> FDLNDFL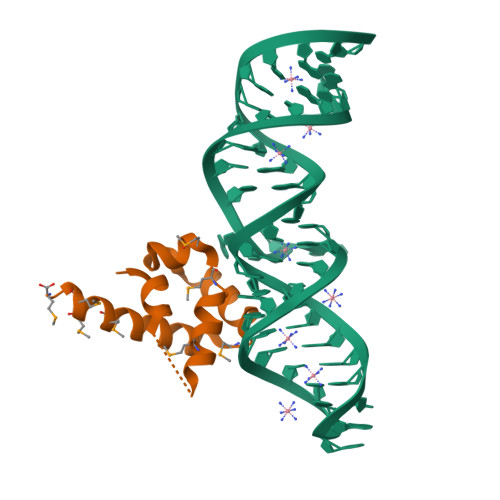EQLRQMKNMGGMASLMGKLPGMGQIPDNVKSQMDDKVLVRMEAIINSMTMKERAKPEIIKGSRKRRIAAGSGMQVQDVNRLLKQFDDMQRMMKKM> MDIFREIASSMKGENVFISPPSISSVLTILYYGANGSTAEQLSKYVEKEADKNKDDISFKSMNKVYGRYSAVFKDSFLRKIGDNFQTVDFTDCRTVDAINKCVDIFTEGKINPLLDEPLSPDTCLLAISAVYFKAKWLMPFEKEFTSDYPFYVSPTEMVDVSMMSMYGEAFNHASVKESFGNFSIIELPYVGDTSMVVILPDNIDGLESIEQNLTDT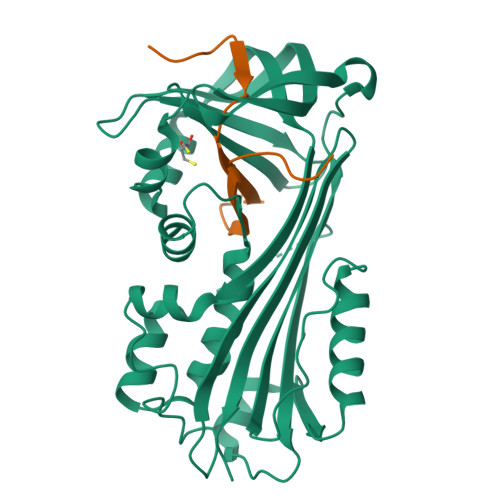NFKKWCDSMDAMFIDVHIPKFKVTGSYNLVDALVKLGLTEVFGSTGDYSNMCNSDVSVDAMIHKTYIDVNEEYTEAAAATCALVADCA;> STVTNEFCADHPFIYVIRHVDGKILFVGRYCSPTTN3-hydroxypropane-1-sulfonic acid | C3 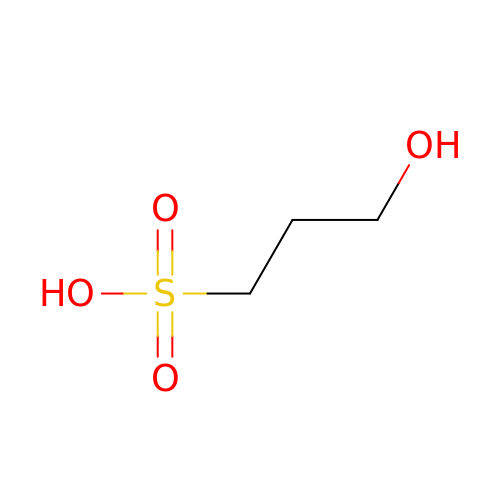H8 O4 S | WQPMYSHJKXVTME-UHFFFAOYSA-N>LRRRYTMVFLPLKWSLATMSFLLSSLLALLTVSTPSWCQSTEASPKRSDGTPFPWNKIRLPEYVIPVHYDLLIHANLTTLTFWGTTKVEITASQPTSTIILHSHHLQISRATLRKGAGERLSEEPLQVLEHPRQEQIALLAPEPLLVGLPYTVVIHYAGNLSETFHGFYKSTYRTKEGELRILASTQFEPTAARMAFPCFDEPAFKASFSIKIRREPRHLAISNMPLVKSVTVAEGLIEDHFDVTVKMSTYLVAFIISDFESVSKITKSGVKVSVYAVPDKINQADYALDAAVTLLEFYEDYFSIPYPLPKQDLAAIPDFQSGAMENWGLTTYRESALLFDAEKSSASSKLGITMTVAHELAHQWFGNLVTMEWWNDLWLNEGFAKFMEFVSVSVTHPELKVGDYFFGKCFDAMEVDALNSSHPVSTPVENPAQIREMFDDVSYDKGACILNMLREYLSADAFKSGIVQYLQKHSYKNTKNEDLWDSMASICPTDGVKGMDGFCSRSQHSSSSSHWHQEGVDVKTMMNTWTLQKGFPLITITVRGRNVHMKQEHYMKGSDGAPDTGYLWHVPLTFITSKSDMVHRFLLKTKTDVLILPEEVEWIKFNVGMNGYYIVHYEDDGWDSLTGLLKGTHTAVSSNDRASLINNA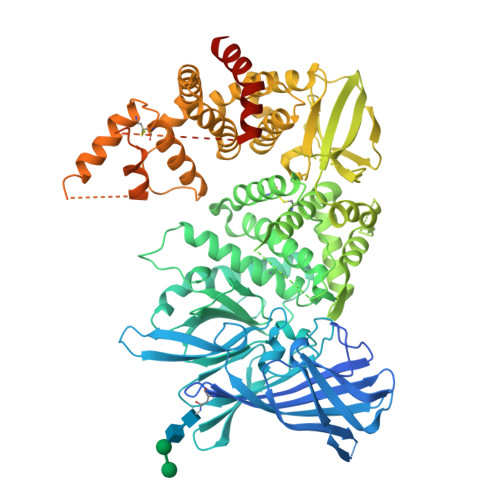FQLVSIGKLSIEKALDLSLYLKHETEIMPVFQGLNELIPMYKLMEKRDMNEVETQFKAFLIRLLRDLIDKQTWTDEGSVSERMLRSQLLLLACVHNYQPCVQRAEGYFRKWKESNGNLSLPVDVTLAVFAVGAQSTEGWDFLYSKYQFSLSSTEKSQIEFALCRTQNKEKLQWLLDESFKGDKIKTQEFPQILTLIGRNPVGYPLAWQFLRKNWNKLVQKFELGSSSIAHMVMGTTNQFSTRTRLEEVKGFFSSLKENGSQLRCVQQTIETIEENIGWMDKNFDKIRVWLQSEKLERMAENLYFQ[3x]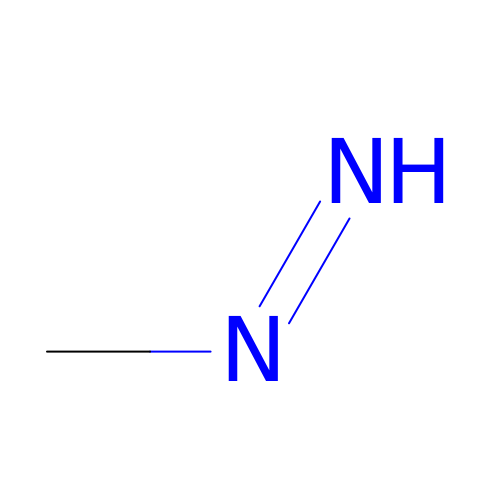METHYLHYDRAZINE | C H4 N2 | JYXPWUYLZPYOAH-IHWYPQMZSA-N> MTRINLTLVSELADQHLMAEYRELPRVFGAVRKHVANGKRVRDFKISPTFILGAGHVTFFYDKLEFLRKRQIELIAECLKRGFNIKDTTVQDISDIPQEFRGDYIPHEASIAIS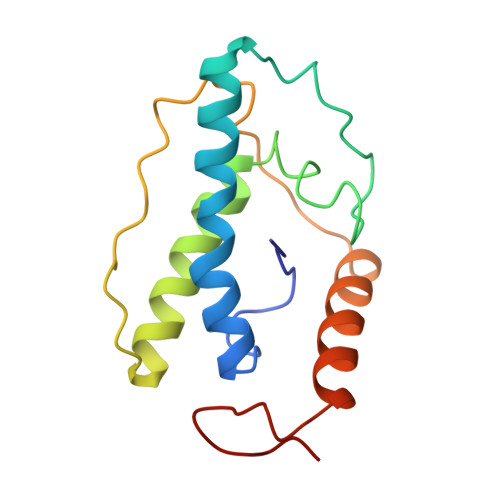QARLDEKIAQRPTWYKYYGKAIYA Bdellovibrio bacteriovorus is a bacterium that preys upon a wide range of other Gram-negative bacteria, entering their periplasm and consuming them from within. Proteomic and structural analyses of vesicle contents reveal several fibre-like proteins, which we name the mosaic adhesive trimer (MAT) superfamily, and show localization on the predator surface before prey encounter. Structural studies reveal a variety of domain usages (and therefore binding capabilities) at the fibre C-termini, placing these on intertwined trimeric β-prisms. Using independent but complementary approaches, we identified and characterized a MAT superfamily of trimeric fibre proteins with diverse adhesive tips, able to fulfil the long-sought-after role of multiplicity of molecular recognition and handling of diverse epitopes (across a wide prey range), by the bacterial predator B. bacteriovorus.

To address the potential for domain-based diversification, we crystallized the tip of Bd1334 (which shares 75% identity with Bd2133 in the fibre region but then diversifies), from S818 and S914 onwards, diffracting to 2.6 Å and 1.4 Å resolution, respectively. The tip of Bd1334 has no similarity to that of Bd2133, forming a β-sandwich of a completely different, square-like shape. Tip trimers are mediated by edge-to-edge contacts, burying 6,900 Å2 per monomer. A composite pocket is formed from two chains, making a tryptophan cage with W1078 and W1102 from one monomer and the terminal W1151 from the opposing monomer. W1102 has an unusual cis peptide bond often enriched in binding sites. There are no structural homologues for Bd1334 in the PDB, and sequence homologues are limited, with sequence conservation patterns being non-informative. Thus, the Bd1334 data show that MAT tips can be swapped out in evolution and that Bd1334 is probably specific for binding an epitope encountered and bound only by B. bacteriovorus bacteria.

> GSAGTLAAPTAVTSGQSLTSLTAFAYNGTQYQSGGNASINFVATEAHTASAGGAKIIFNTTNNGATGSTEKVVIDQNGNVGVGVGAPTAKMDVNGGIKQPNYGIISAVRNSGGVTASMPWTNAYVLAHQGEMHQWVAGGPILQDSVTGCNAGPDAGVKFDSIATSWGGPYKVIFHTTGSNGAIHLEWSGWQVSLKNSAGTELAIGMGQVFATLHYDPAVSNWRVEHMFGRINNTNFTCW>[4x]DREKIYQWINELSSPETRENALLELSKKRESVPDLAPMLWHSFGTIAALLQEIVNIYPSINPPTLTAHQSNRV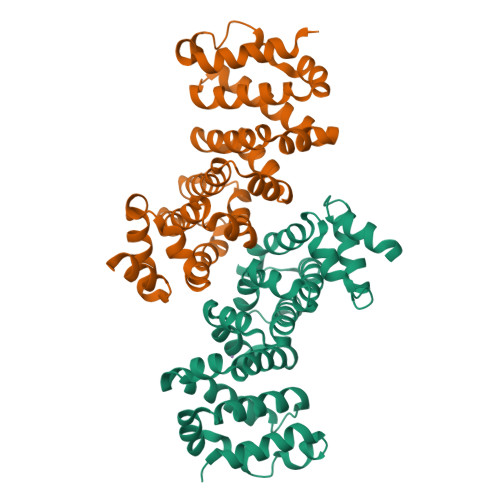CNALALLQCVASHPETRSAFLAAHIPLFLYPFLHTVSKTRPFEYLRLTSLGVIGALVKTDEQEVINFLLTTEIIPLCLRIMESGSELSKTVATFILQKILLDDTGLAYICQTYERFSHVAMILGKMVLQLSKEPSARLLKHVVRCYLRLSDNPRAREALRQCLPDQLKDTTFAQVLKDDTTTKRWLAQLVKNLQE> SMPKTISVRVTTMDAELEFAIQPNTTGKQLFDQVVKTIGLREVWFFGLQYQDTKGFSTWLKLNKKVTAQDVRKESPLLFKFRAKFYPEDVSEELIQDITQRLFFLQVKEGILNDDIYCPPETAVLLASYAVQSKYGDFNKEVHKSGYLAGDKLLPQRVLEQHKLNKDQWEERIQVWHEEHRGMLREDAVLEYLKIAQDLEMYGVNYFSIKNKKGSELWLGVDALGLNIYEQNDRLTPKIGFPWSEIRNISFNDKKFVIKPIDKKAPDFVFYAPRLRINKRILALCMGNHELYMRRRKPDTIEVQQMKAQAR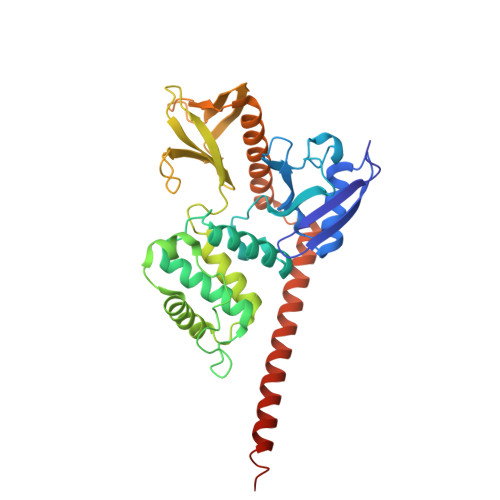EEKHQKQMERAMLENEKKKREMAEKEKEKIEREKEE N~1~-(5-chloro-1H-imidazo[4,5-b]pyridin-2-yl)-N~2~-[(4R)-6,8-dichloro-1,2,3,4-tetrahydroquinolin-4-yl]-N~1~-methylethane-1,2-diamine | C18 H19 Cl3 N6 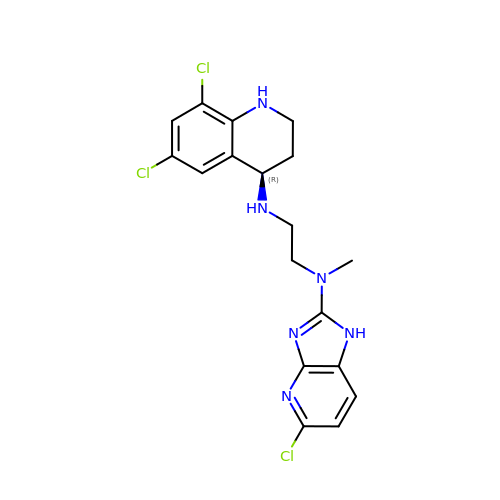| XBDCSRQKOZIJKF-CYBMUJFWSA-N>[2x]MTPVAEGGLPHGSVPSLSHTRQWRPGVVQEVAPAGVLDLGPGYIEPALLPVRLLRGAYEQALAEYGAAALGYGHDPGAQPLRDRLAARAAAADGLPCDPDQVLLTS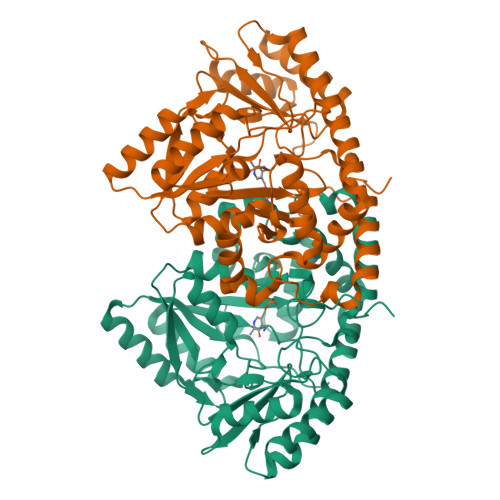GTSQALYLLATSLAAPGDTVLTEELCYDLGQRIFRDCSLRLRQVAMDGSGMLPDALDRALTEGARAGAKTAFVYLTPTHHNPTGHTMPLARRRLLLEVAARHDVLIVEDDAYTELSLIPDRTPPPSLAALAGYRRVVRLCSFSKTLGPGLRLGWLLADRELAGRLATHGLFVSGGSLNHTTSLAVSTLLASGAYDRHLDAFRAQLRARRDALVGALRAMLDDGVELRTPEGGFFLWLRAGDGADERELLDGAARAGVRIAAGSRFGTTQGAGLRLAFSFNPPALLEQAAKRLTTAWSGSTPDLEIGVRS> DALKPEDKVKFRQASYTTMAWNMGKIKAMVVDGTMPFSQTQVSAAANVIAAIANSGMGALYSPDTLGVVGFKKSRLKENFFQEQDEVRKIATNFVEQANKLAEVAAMGDKDEIKAQFGEVGKACKACHEKFREEE

Here, the current status of the fully automated ambient-temperature beamline VMXi at Diamond Light Source is described, and a highly efficient pipeline from protein sample to final multi-crystal data analysis and structure determination is shown. The VMXi beamline and its associated PXF within the Research Complex at Harwell offer a highly automated pipeline where researchers provide a suitable protein sample that is used for robotic crystallization, monitoring and subsequent in situ data collection from crystals in crystallization plates or in thin-film sample delivery systems. Here we present illustrative examples of data measured using VMXi from a variety of proteins comprising both conventional crystallographic standards and ‘real world’ user samples. Routine RT data collection provides a useful capability that is highly relevant to studying protein dynamics and ligand binding without the complication of cryo-cooling.

Other users tend to focus on groups of proteins with homologous functions from a range of microorganisms. This is the case of a group working with cytochromes c′. Furthermore, they pose a challenge as their heme centre is very sensitive to radiation, and thus careful data collection and analysis are crucial. For the α-helical cytochrome c′ protein from H. thermoluteolus (PHCP), a total of two plates were set up yielding one crystal hit for the PHCP protein under the 96 screening conditions. A structure at 1.88 Å resolution was determined from four data wedges, each of 60°, measured at different positions on a single larger crystal. Notably, because of the high-symmetry space group (P6222), a single 60° wedge gave a 2.08 Å dataset with 99.4% complete­ness, but adding the three further wedges within xia2.multiplex increased completeness to 100% and led to a significant improvement in dataset resolution. In this case, only a single crystal was required for RT structure determination because of the high-symmetry crystal form and the ability to measure data from multiple positions along the crystal. The overall RT PHCP structure showed a four-helix bundle, superimposing well with the cryo-structure having an RMSD value of 0.38 Å.> MVEDILAPGLRVVFCGINPGLSSAGTGFPFAHPANRFWKVIYQAGFTDRQLKPQEAQHLLDYRCGVTKLVDRPTVQANEVSKQELHAGGRKLIEKIEDYQPQALAILGKQAYEQGFSQRGAQWGKQTLTIGSTQIWVLPNPSGLSRVSLEKL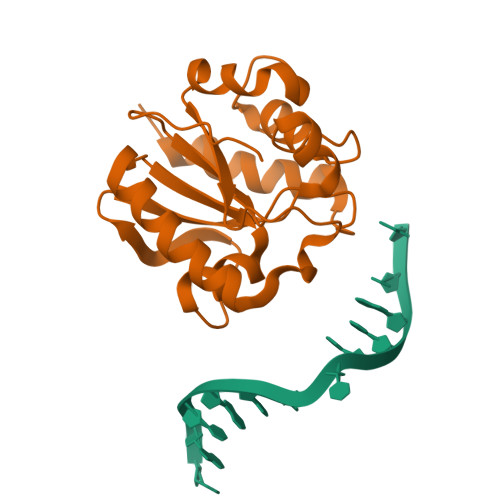VEAYRELDQALVVRGR>[3x]M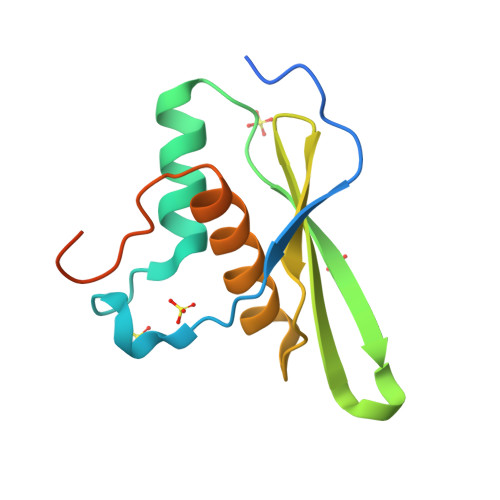TSEQTGEPAEDTSGVIKMAVKFDRRAYPAQITPKMCLLEWCRREKLAQPVYETVQRPLDRLFSSIVTVAEQKYQSTLWDKSKKLAAQAAAIVCLRSQGLPEGRLGEESPSLHKHHHHHH>[2x]MALTAALKAQIAAWYKALQEQIPDFIPRAPQRQMIADVAKTLAGEEGRHLAIEAPTGVGKTLSYLIPGIAIAREEQKTLVVSTANVALQDQIYSKDLPLLKKIIPDLKFTAAFGRGRYVCPRNLTALASTEPTQQDLLAFLDDELTPNNQEEQKRCAKLKGDLDTYKWDGLRDHTDIAIDDDLWRRLSTDKASCLNRNCYYYRECPFFVARREIQEAEVVVANHALVMAAMESEAVLPDPKNLLLVLDEGHHLPDVARDALEMSAEITAPWYRLQLDLFTKLVATCMEQFRPKTIPPLA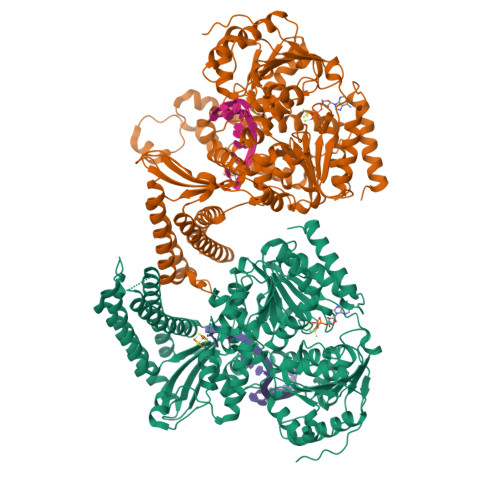IPERLNAHCEELYELIASLNNILNLYMPAGQEAEHRFAMGELPDEVLEICQRLAKLTEMLRGLAELFLNDLSEKTGSHDIVRLHRLILQMNRALGMFEAQSKLWRLASLAQSSGAPVTKWATREEREGQLHLWFHCVGIRVSDQLERLLWRSIPHIIVTSATLRSLNSFSRLQEMSGLKEKAGDRFVALDSPFNHCEQGKIVIPRMRVEPSIDNEEQHIAEMAAFFREQVESKKHLGMLVLFASGRAMQRFLDYVTDLRLMLLVQGDQPRYRLVELHRKRVANGERSVLVGLQSFAEGLDLKGDLLSQVHIHKIAFPPIDSPVVITEGEWLKSLNRYPFEVQSLPSASFNLIQQVGRLIRSHGCWGEVVIYDKRLLTKNYGKRLLDALPVFPIEQPEVPEGIVKKKEKTKSPRRRRR> GDEKQFQIEKWQIARC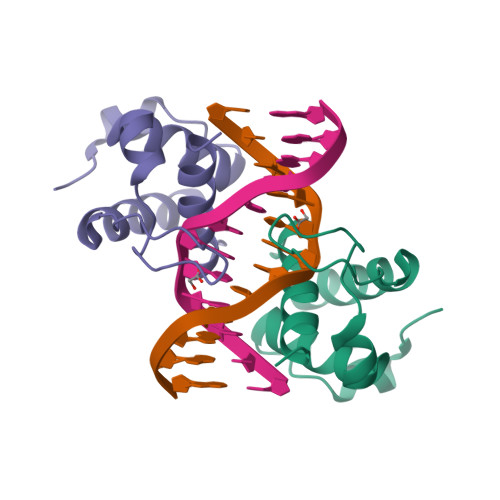NKSKPQKFINDLMQVLYTNEYMATHSLTGAKSSTSRDKAVKPAMNQNEVQEIIGVTKQLFPNTDDVSIRRMIGQKLNNCTKKPNLSK3-[[6-tert-butyl-2-[methyl-[(3S)-1-methylpyrrolidin-3-yl]amino]thieno[3,2-d]pyrimidin-4-yl]-methyl-amino]propanenitrile 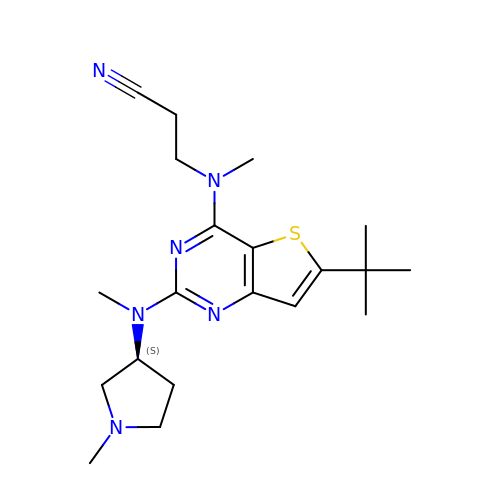| C20 H30 N6 S | IIIBKWKCKFKYOT-AWEZNQCLSA-N> MPRLTTITLYEHDEKRYRDIAGDKKAIQDALIKLNKQFKKDFKKLDRSEDNSDTEDTIDE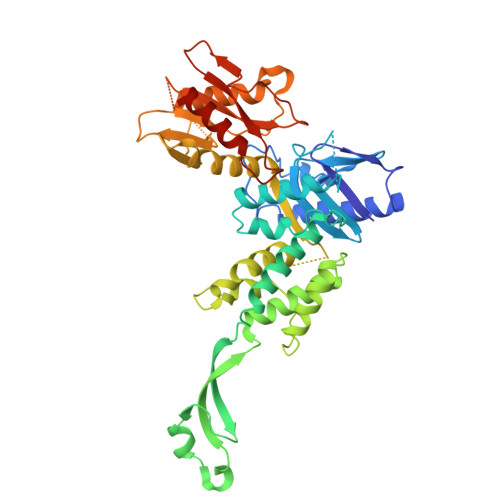SKGVVEVYANKIKARHYVGFAAVDNVFLQILPKVFKPKKEQTQETQEDTWEPILAFIRMLDMAYGLKIKDHDLAYLQGRNLRPNLYEVFIYLFAKSLWSEVQRGYHREYVEVHREEKFLRGKLLMSRQIRKLPHQLNTFSVEVHELIEDNLLNRIFYASVREALRRTTWGLNRKLLGELMLAFDGITPIHLRTEHFERVHFTRLNERFRRPFELAKLLFMPASGKGRSREVSGFFVDMNKLFERFIERVLVRNLPPEYKLFYQESYPFLKNQNGSSQKPDYVVRKGNTPVVVLDAKYRELKERIPSSDMLRQLYVYSRIWGYKTSHENDSKPPAVIVIPSSSTYNQGLPDKPLEFEFFDERKLFIVAYNMDYVKTGAIFKADKNFRRSLNNIIGKLNT Aprataxin, aprataxin and PNKP-like factor (APLF) and polynucleotide kinase phosphatase (PNKP) are key DNA-repair proteins with diverse functions but which all contain a homologous forkhead-associated (FHA) domain. Their primary binding targets are casein kinase 2-phosphorylated forms of the XRCC1 and XRCC4 scaffold molecules which respectively coordinate single-stranded and double-stranded DNA break repair pathways. The precise role of APLF is yet to be determined although it does possess both endo- and exo-nuclease activity and its depletion is associated with impairment of NHEJ. These three proteins share highly homologous forkhead-associated (FHA) domains, which have been shown to function as protein–protein interaction modules through their specific recognition of phosphothreonine-containing motifs on interacting partners.

Here, we present the high-resolution X-ray structure of a complex of phosphorylated XRCC4 with APLF, the most divergent of the three FHA domain family members. The final model contains two complexes each comprising residues 1–104 of APLF with an additional five N-terminal-residues derived from the cleaved GST-tag and the bound tri-phosphorylated XRCC4 phosphopeptide. Comparison of the APLF FHA domain structure with those of PNKP and aprataxin shows that, as expected from the relatively high degree of sequence homology, their FHA domain β-sandwich folds are similar overall, although, consistent with sequence comparison, the APLF structure is most divergent and contains a six-residue extension in loop β6–β7. The XRCC4 phosphopeptide adopts an orientation similar to that observed in previously reported FHA/phosphopeptide structures, lying across the tips of loops β3–β4 and β5–β6. A second set of hydrogen bonds constrains the peptide backbone on either side; the Arg27 side-chain interacts with the pT −2 and the Asn60 side-chain hydrogen-bonds with the pT +1 carbonyl. Tyr229 in position pT −4 is held in place by a hydrophobic stacking interaction with Pro29. In accordance with the lack of binding effect associated with phosphorylation of Ser237, only residues pT −4 to pT +2 could be modelled into the electron density, indicating that the C-terminal end of the peptide, including Asp236 at pT +3, and pSer237 at the pT +4 position, is mobile. Side-chain density for APLF Lys36, equivalent to PNKP Arg44 is very poor suggesting that it is highly mobile. However, it appears to be in a suitable position for electrostatic recognition of both Glu pT −2, Asp pT +1 and pSer at pT −1 (see below). Interestingly, in the APLF/XRCC4 structure the pT −1 phosphoserine assumes an upright, solvent exposed conformation, making no direct contacts to FHA domain residues.

>[2x]GPLGSMSGGFELQPRDGGPRVALAPGETVIGRGPLLGITDKRVSRRHAILEVAGGQLRIKPIHTNPCFYQSSEKSQLLPLKPNLWCYLNPGDSFSMLVDKYIFRILSIPSA;>AYDESTDEE[2x]> ESKEGSRSSKAKLQISVARSERLLREHGGCSRVSEGAAVALAAAIEYFMGEVLELAGNAARDSKKVRISVKHITLAIQNDAALFAVVGKGVFSGAGVSLISVP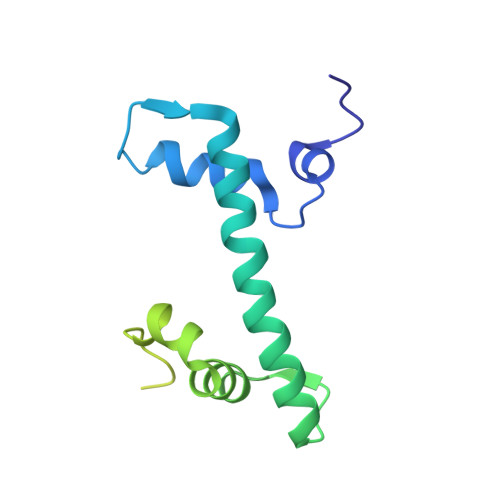IPRKKARKTTEKEASSPKKKAAPKKKKAASKQKKSLSDKELAKLTKKELAKYEKEQGMSPGY> NYKKPKLLYCSNGGHFLRILPDGTVDGTRDRSDQHIQLQLSAESVGEVYIKSTETGQYLAMDTDGLLYGSQTPNEE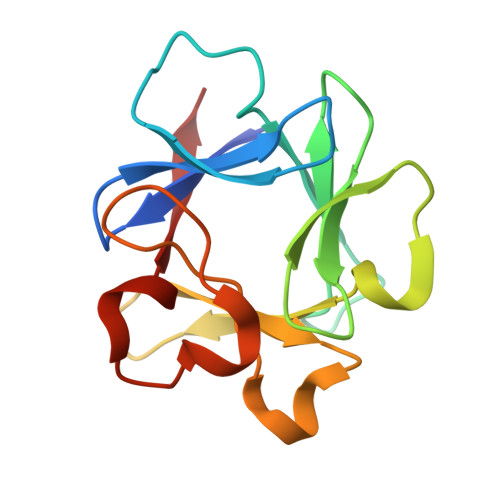CLFLERLEENHYNTYISKKHAEKNWFVGLKKNGSCKRGPRTHYGQKAILFLPLPV> MERNKLARQIIDTCLEMTRLGLNQGTAGNVSVRYQDGMLITPTGIPYEKLTESHIV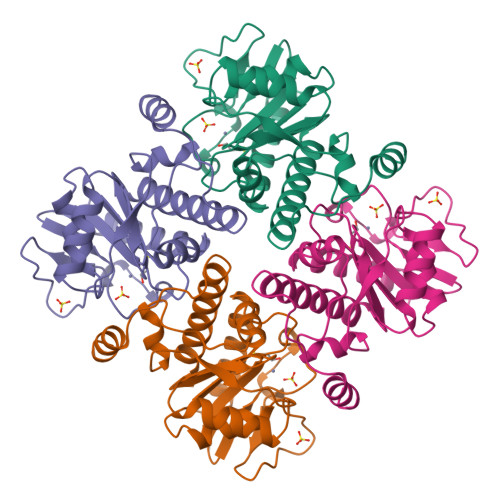FIDGNGKHEEGKLPSSEWRFHMAAYQSRPDANAVVHNHAVHCTAVSILNRSIPAIHYMIAAAGGNSIPCAPYATFGTRELSEHVALALKNRKATLLQHHGLIACEVNLEKALWLAHEVEVLAQLYLTTLAITDPVPVLSDEEIAVVLEKFKTYGLRIEE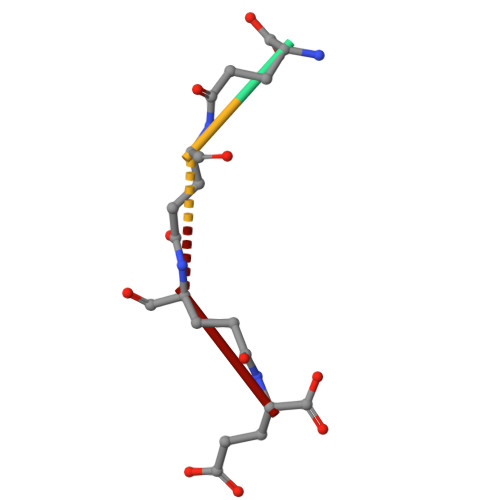> EEEE>[6x]GSHMGHSMDSLIAQCSPEADTLLTDNPSKANRILEDPDYSLVKALQMAQQNFVITDASLPDNPIVYASRGFLTLTGYSLDQILGRNCRF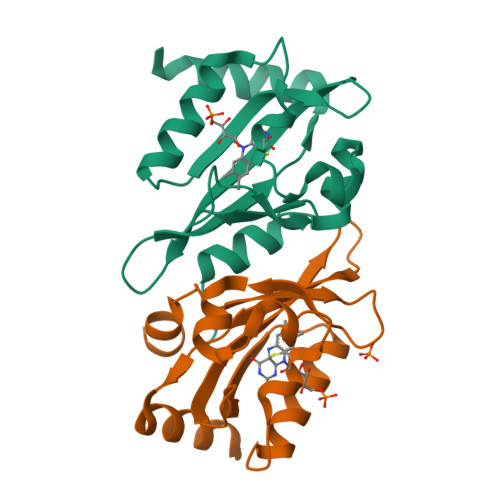LQGPETDPRAVDKIRNAITKGVDTSVCLLNYRQDGTTFWNLFFVAGLRDSKGNIVNYVGVQSKVSEDYAKLLVNEQNIEYK Ferritin from the marine pennate diatom Pseudo-nitzschia multiseries (PmFTN) plays a key role in sustaining growth in iron-limited ocean environments. Typically formed from 24 subunits arranged as a symmetric, hollow sphere, ferritins take up soluble Fe2+ and catalyze its oxidation, with the resulting Fe3+ being stored as an oxy-hydroxide mineral in its central cavity. The di-iron catalytic ferroxidase center of PmFTN (sites A and B) has a nearby third iron site (site C) in an arrangement typically observed in prokaryotic ferritins. Here we demonstrate that Glu-44, a site C ligand, and Glu-130, a residue that bridges iron bound at sites B and C, limit the rate of post-oxidation reorganization of iron coordination and the rate at which Fe3+ exits the ferroxidase center for storage within the mineral core.

Two structures were obtained from E44H PmFTN crystals soaked for 45 min (E44H Fe (45 min)) and 3 h (E44H Fe (3 h)) in aerobic Fe2+ solution. All three sites are occupied by iron ions with modest differences in metal occupancy regardless of the crystal soaking time. These structures revealed that the coordination spheres of the iron ions in sites A, B, and C are markedly altered in the E44H variant relative to the wild type PmFTN structure, exhibiting what might be described as ligand scrambling. The side chain conformation of His-51 is altered such that this residue now coordinates to the iron at site C (Fe-C) rather than Fe-A, which is thus coordinated only by Glu-15, Glu-48, a water molecule, and the bridging water or oxo/hydroxo group. His-44 and Glu-130 are ligands of Fe-B. Fe-C is coordinated by His-51 and Glu-130 and forms weaker interactions with Gln-126 and Glu-47. A water molecule is observed bridging Fe-C and Fe-B. As a result of these differences, Fe-C is displaced toward site A by ∼3.5 Å as compared with wild type PmFTN and the E44Q variant. Structural data showed that, in both cases, iron at one of the sites (Fe-B in E130A PmFTN and Fe-A in E44H PmFTN) has fewer ligands than in the wild type structure, suggesting that inequivalent Fe2+ affinity at Fe-A and Fe-B accounts for the loss of positive cooperativity. E44Q PmFTN has a rate constant ∼6-fold higher than that of wild type, whereas the rate constant for E44H PmFTN is about 3-fold lower than that of wild type PmFTN. Mineralization in E44Q PmFTN was similar to wild type protein (initial rates of 7.0 ± 0.9 and 4.1 ± 0.8 μm Fe2+ min−1, respectively), whereas mineralization in E44H PmFTN was significantly slower (1.7 ± 0.5 μm Fe2+ min−1).

>GSEELLDLFNRQVTQEFTASQVYLSASIWFDQNDWEGMAAYMLAHSAEEREHGLGFVDFANKRNIPIELQAVPAPVSCAEWSSPEDVWQSILELEQANTRSLLNLAEAASTCHDFAVMAFLNPFHLQQVNEEDKIGSILAKVTDENRTPGLLRSLDVVSFLGPCLFRSV[6x]> MPKRH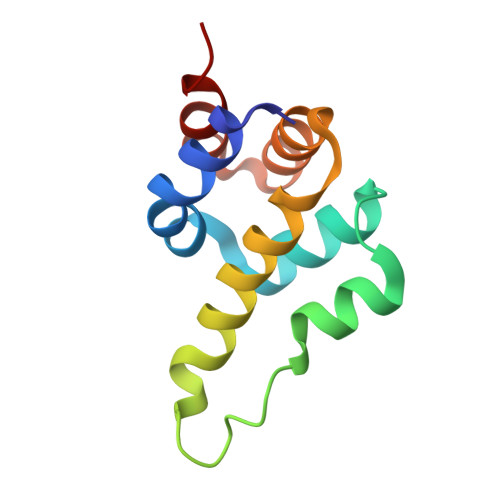REHIRKNLNILVEWTNYERLAMECVQQGILTVQMLRNTQDLNGKPFNMDEKDVRVEQHRRLLLKITQRGPTAYNLLINALRNINCLDAAVLLESVDE> ATVLLEVPFSARGDRIPDAVAELRTREPIRKVRTITGAEAWLVSSYALCTQVLEDRRFSMKETAAAGAPRLNALTVPPEVVNNMGNIADAGLRKAVMKAITPKAPGLEQFLRDTANSLLDNLITEGAPADLRNDFADPLATALHCKVLGIPQEDGPKLFRSLSIAFMSSADPIPAAKINWDRDIEYMAGILENPNITTGLM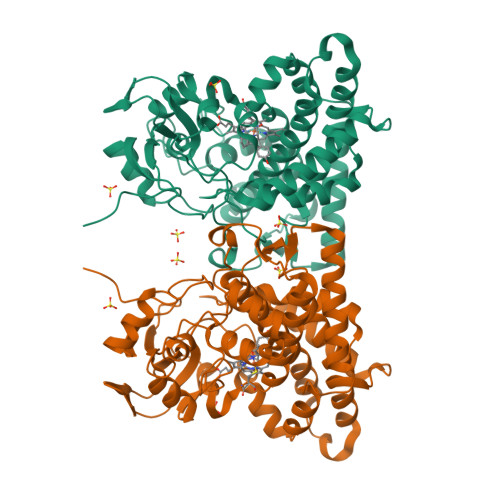GELSRLRKDPAYSHVSDELFATIGVTFFGAGVISTGSFLTTALISLIQRPQLRNLLHEKPELIPAGVEELLRINLSFADGLPRLATADIQVGDVLVRKGELVLVLLEGANFDPEHFPNPGSIELDRPNPTSHLAFGRGQHFCPGSALGRRHAQIGIEALLKKMPGVDLAVPIDQLVWRTRFQRRIPERLPVLW>MATDLKASSLRALKLMHLATANGDDTDEKVIALCHQAKTPVGTTDAIFIYPRFIPIARKTLKEQGTPEIRIWTSTNFPHGNDDIDIALAETR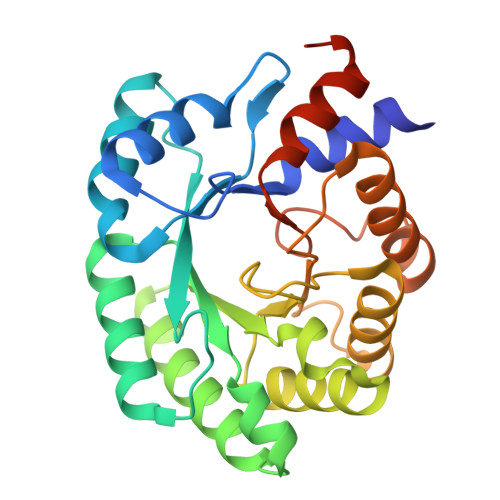AAIAYGADGVAVVFPYRALMAGNEQVGFDLVKACKEACAAANVLLSVIIETGELKDEALIRKASEISIKAGADHIVTSTGKVAVGATPESARIMMEVIRDMGVEKTVGFIPAGGVRTAEEAQKYLAIADELFGADWADARHYAFGASSLLASLLKALGYGDGKSASSYGSLE[2x]>[2x]MVLYFIGLGLYDERDITVKGLEIAKKCDYVFAEFYTSLMAGTTLGRIQKLIGK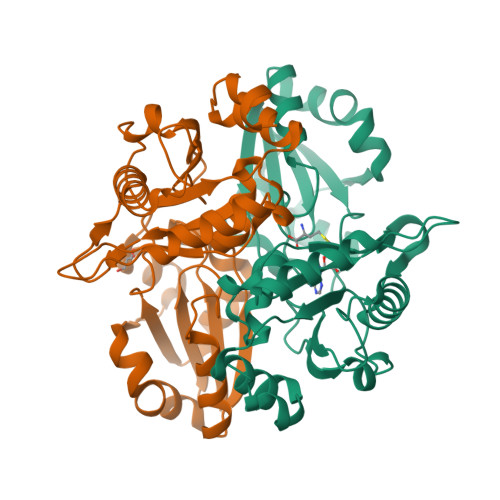EIRVLSREDVELNFENIVLPMAKENDVAFLTPGDPLVATTHAELRIRAKRAGVESYVIHAPSIYSAVGITGLHIYKFGKSATVAYPEGNWFPTSYYDVIKENAERGLHTLLFLDIKAEKRMYMTANEAMELLLKVEDMKKGGVFTDDTLVVVLARAGSLNPTIRAGYVKDLIREDFGDPPHILIVPGKLHIVEAEYLVEIAGAPREILRVNV>GPMGKMAAAVASLATLAAEPREDAFRKLFRFYRQSRPGTADLGAVIDFSEAHLARSPKPGVPQVVRFPLNVSSVTERDAERVGLEPVSKWRAYGLEGYPGFIFIPNPFLPGCQRHWVKQCLKLYSQKPNVCNLDKHMTKEETQGLWEQSKEVLRSKEVTKRRPRSLLERLRWVTLGYHYNWDSKKYSADHYTPFPSDLAFLSEQVATACGFQGFQAEAGILN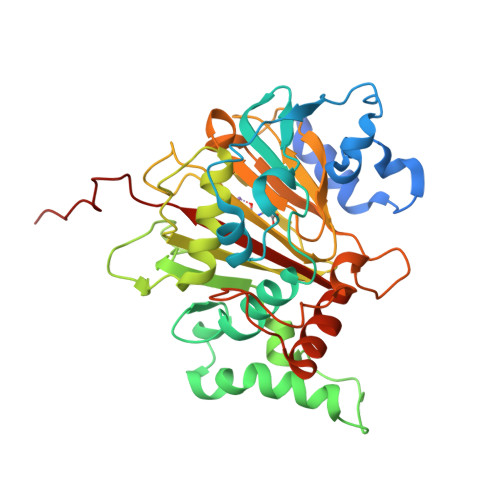YYRLDSTLGIHVDRSELDHSKPLLSFSFGQSAIFLLGGLKRDEAPTAMFMHSGDIMVMSGFSRLLNHAVPRVLPHPDGECLPHCLETPLPAVLPSNSLVEPCSVEDWQVCATYLRTARVNMTVRQVLATGQDFPLEPVE[4x]> TAGAAWACFRLDGRTLLRVRGPDAAPFLLGLLTNELPLPSPAAAGAPPAARAGYAHFLNVQGRTLYDVILYGLQEHSEVSGFLLECDSSVQGALQKHLALYRIRRKVTVEPHPELRVWAVLPSSP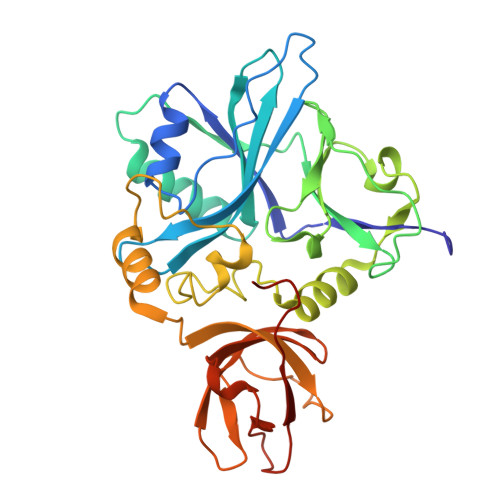EACGAASLQERAGAAAILIRDPRTARMGWRLLTQDEGPALVPGGRLGDLWDYHQHRYLQGVPEGVRDLPPGVALPLESNLAFMNGVSFTKGAYIGQELTARTHHMGVIRKRLFPVRFLDPLPTSGITPGATVLTASGQTVGKFRAGQGNVGLALLWSEKIKGPLHIRASEGAQVALAASVPDWWPTVSK> EVDKRREINNEHPLLMMPLYANGEEFNQGKYTFWGGDTLTGKWENIPDDLKPYTVIQLHPDDLPKRDGAARDFYEHMLEEAAKYVNPKTGKNEPIPVILTVYTAGNMPYYTSAHWLSTSWIDKMYQKYPNLHGIFSTASYWIWANDIENKAADYLKVSAKNGGYFIWAEQNSGSAIEKAFGKNGKIAFQKSVDKYWKNLIFMFKNTPAAEGNDSTTESYMKGLWLSNHTYQWGGLMDTWKWYETGKWKLFASGNIGKSQGDRQWLTEPESMLGEEALGVYLNGGVVYNFEHPAYTYGVNNKESLLFSEVIKEFFRYVIAHPAPSKEKVLEDTKVFIHGDYSNKGNGKFFVNVNTDREQTPLYMTGRYNVIPAIPGVLKTDKL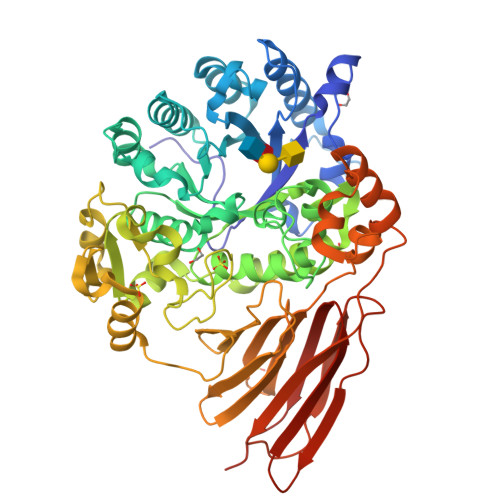KESVSSSRIQIKEITSPEFSSTQARKEYLNKLYPMNYEGDIFAQKLDNRWFVYNYKVNENVKQTGKLKFNSLEMNVEFEPHTYGIFERISNGLKVNLNNFRTNKDSLWSNAQDANQAKKLPQLTKKGAIKWIEEHYIKDTQFGEKRVTKIVLRGIDKLPTIHSLSGTNNSYDQPSLNFDQKNHMVTITINSNGNLEFELHFLEHTRAPPPPPLRSGC> HHHHHHGSMLQKAIRQQQQHYLSDEFNFVTL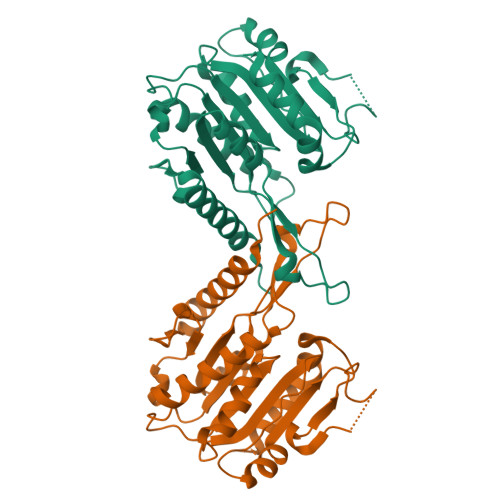PLVSMDLPDNTVLCTPNISESNTIIIVVHDTSDIWAKRNVISGTIDLSSSVIIDNSLDFIKWGLDRKYGIIDVNIPLTLFEPDNYSGMITSQEVLIYLWDNYIKYFPSVAKIAFIGIGDSYSGIVHLLGHRDTRAVTKTVINFLGDKQLKPLVPLVDETLSEWYFKNSLIFSNNSHQCWKENESRKPRKKFGRVLRCDTDGLNNIIEERFEEATDFILDS>GSHMDYNKRSSVSTVPNAAPIRVGFVGLNAAKGWAIKTHYPAILQLSSQFQITALYSPKIETSIATIQRLKLSNATAFPTLESFASSSTIDMIVIAIQVASHYEVVMPLLEFSKNNPNLKYLFVEWALACSLDQAESIYKAAAERGVQTIISLQGRKSPYILRAKELISQGYIGDINSIEIAGNGGWYGYERPVKSPKYIYEIGNGVDLVTTTFGHTIDILQYMTSSYFSRINAMVFNNIPEQELIDERGNRLGQRVPKTVPDHLLFQGTLLNGNVPVSCSFKGGKPTKKFTKNLVIDIHGTKGDLKLEGDAGFAEISNLVLYYSGTRANDFPLANGQQAPLDPGYDAGKEIMEVYHLRNYNAIVGNIHRLYQSISDFHFNTKKIPELPSQFVMQGFDFEGFPTLMDALILHRLIESVYKSNMMGSTLNVSNISHYSL[2x];>[2x]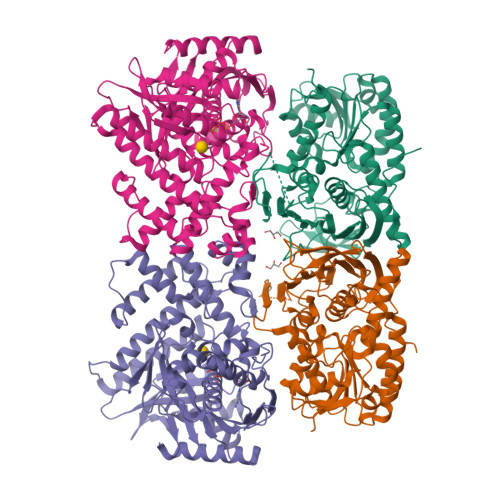SNTNVPIFSSPVRDLPRSFEQKHLAVVDAFFQTYHVKPDFIARSPGRVNLIGEHIDYCDFSVLPLAIDVDMLCAVKILDEKNPSITLTNADPKFAQRKFDLPLDGSYMAIDPSVSEWSNYFKCGLHVAHSYLKKIAPERFNNTPLVGAQIFCQSDIPTGGGLSSAFTCAAALATIRANMGKNFDISKKDLTRITAVAEHYVGVNNGGMDQATSVYGEEDHALYVEFRPKLKATPFKFPQLKNHEISFVIANTLVKSNKFETAPTNYNLRVIEVTVAANALATRYSVALPSHKDNSNSERGNLRDFMDAYYARYENQAQPWNGDIGTGIERLLKMLQLVEESFSRKKSGFTVHEASTALNCSREEFTRDYLTTFPVRFQVLKLYQRAKHVYSESLRVLKALKMMTSATFHTDEDFFTDFGRLMNESQASCDKLYECSCIETNQICSIALANGSFGSRLTGAGWGGCTIHLVPSGANGNVEQVRKALIEKFYNVRYPDLTDEELKDAIIVSKPALGTCLYEQ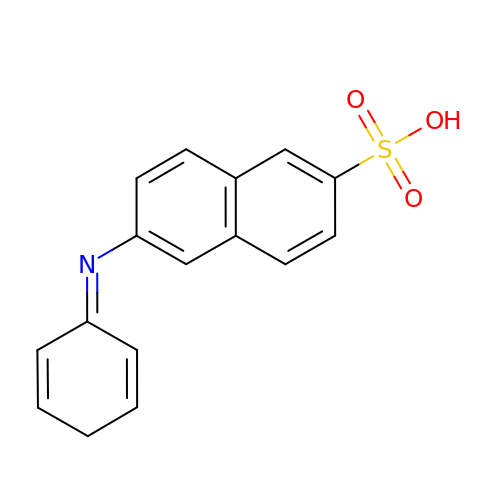6-[(1E)-CYCLOHEXA-2,4-DIEN-1-YLIDENEAMINO]NAPHTHALENE-2-SULFONATE | C16 H13 N O3 S | WXUMRSOAQINBNG-UHFFFAOYSA-N>MKILVIEDDALLLQGLILAMQSEGYVCDGVSTAHEAALSLASNHYSLIVLDLGLPDEDGLHFLSRMRREKMTQPVLILTARDTLEDRISGLDTGADDYLVKPFALEELNARIRALLRRHNNQGDNEISVGNLRLNVTRRLVWLGETALDLTPKEYALLSRLMMKAGSPVHREILYNDIYSGDNEPATNTLEVHIHNLREKIGKSR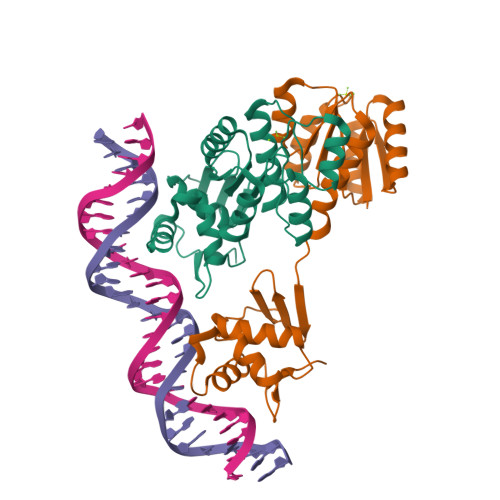IRTVRGFGYMLANNDDTEHLEHHHHHH[2x]> HMGTGSLGGGFPGKGMKIVTSFYPIYAMVKEVSGDLNDVRMIQSSSGIASFEPSANDIAAIYDADVFVYHSHTLESWAGSLDPNLKKSKVKVLEASEGMTLERVPGLEDVEAGDGVDEKTLYDPHTWLDPEKAGEEAQIIADKLSEVDSEHKETYQKNAQAFIKKAQELTKKFQPKFEKATQKTFVTQHTAFSYLAKRFGLNQLGIAGISPEQEPSPRQLTEIQEFVKTYKVKTIFTESNASSKVAETLVKSTGVGLKTLNPLESDPQNDKTYLENLEENMSILAEELKGNLYFQ

Streptococcus pneumoniae scavenges essential zinc ions from the host during colonization and infection. This is achieved by the ATP-binding cassette transporter, AdcCB, and two solute-binding proteins (SBPs), AdcA and AdcAII. AdcAII belongs to the cluster A-I subgroup of SBPs, consisting of a conserved structural fold of two (β/α)4 domains connected by a rigid α-helix, with the metal-binding site located at the interface between the N- and C-terminal lobes (Loisel et al., 2008; Yukl, 2017).

In this study, we investigated the Zn(II)-binding mechanism of AdcAII by mutating each of the four Zn(II)-coordinating residues in the SBP. Structural analyses of Zn(II)-bound AdcAII variants revealed that specific regions within the protein underwent conformational changes via direct coupling to each of the metal-binding residues. The binding site mutations impacted protein conformation and interaction with Zn(II) to differing extents. Quantitative in vitro metal-binding assays combined with affinity determination and phenotypic growth assays revealed that each of the four Zn(II)-coordinating residues contributes to metal binding by AdcAII. Intriguingly, the phenotypic growth impact of the mutant adcAII alleles was, in general, independent of affinity, suggesting that the Zn(II)-bound conformation of the SBP is crucial for efficacious metal uptake. Taken together, these data demonstrate the importance of SBP-metal complex conformation for bacterial Zn(II) uptake.>[2x]MAEIPLFPLSNALFPAGVLRLRVFEIRYLDMVRRCIADGSEFGVVVLEQGT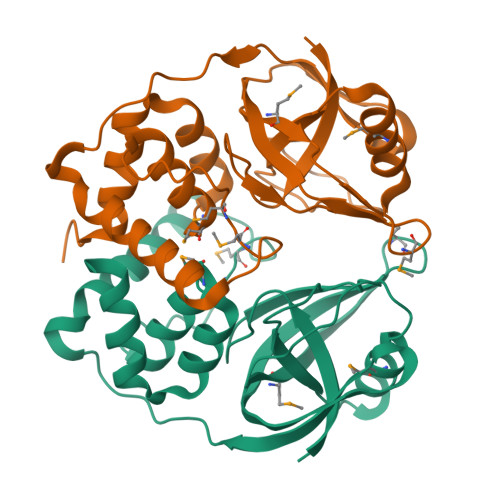EVRRPDGREVLARAGTMARIDHWEAPMPALLELACTGTGRFRLHACTQGKYGLWTGQAEPVPDDAPLEVPPELARSASALGRLIARLQREGVPPHIMPMAAPFRLDDCGWVADRWAEMLSLPPADKARLLLLPPLDRLREIDAVLAADGHALEHHHHHH6-[4-(benzyloxy)phenyl]-1-(pyridin-4-ylmethyl)-1H-pyrazolo[3,4-b]pyridine-4-carboxylic acid | C26 H20 N4 O3 | 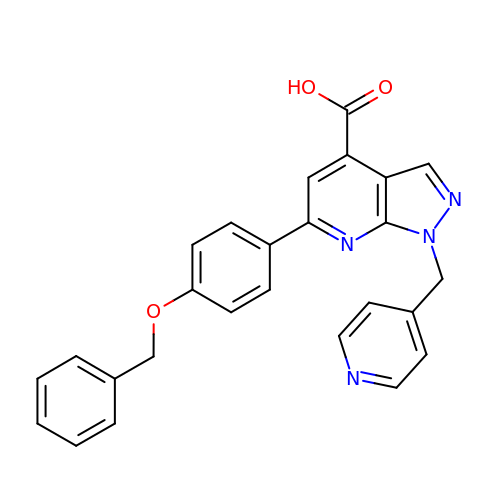LEKPQTJLNDALBT-UHFFFAOYSA-N> QDNSRYTHFLTQHYDAKPQGRDDRYC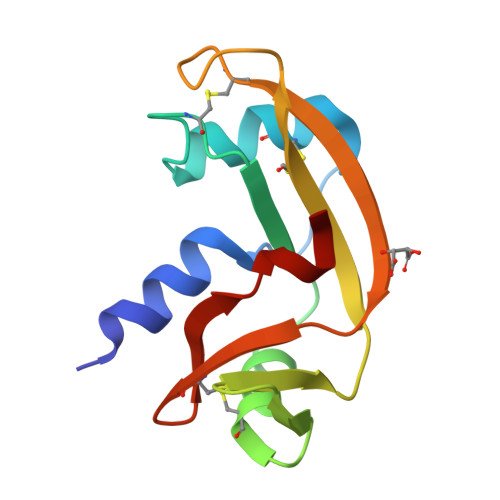ESIMKRRGLTSPCKDINTFIHGNKRSIKAICENKNGNPHRENLRISKSSFQVTTCKLHGGSPWPPCQYRATAGFRNVVVACENGLPVHLDQSIFRRP>SMQEGSLPDITIFPNSSLMISQGTFVTVVCSYSDKHDLYNMVRLEKDGSTFMEKSTEPYKTEDEFEIGPVNETITGHYSCIYSKGITWSERSKTLELKVIKE[4x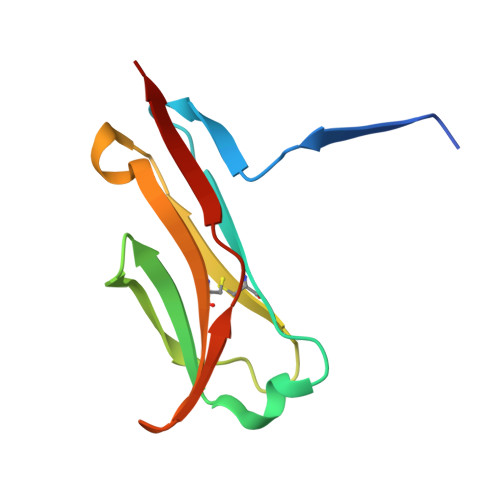]> GMDEIVKNIREGTHVLLPFYETLPELNLSLGKSPLPSLEYGANYFLQISRVNDLNRMPTDMLKLFTHDIMLPESDLDKVYEILKINSVKYYGRTTRADAVVADLSARNKLFKRERDAIKSNNHLTENNLYISDYKMLTFDVFRPLFDFVNEKYCIIKLPTLFGRGVIDTMRIYCSLFKNVRLLKCVSDSWLKDSAIMVASDVYKKNLDLFMSHVKSVTKSSSWKDVNTVQFSILNDPVDTEFTNKFLEFSNRVYEALYYVHSLLYSSMTSDSKSIENK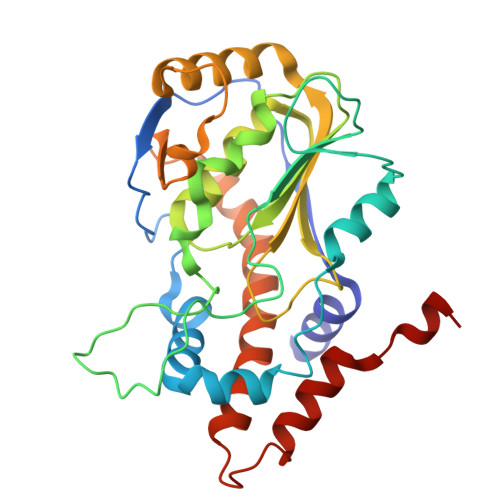HQRRLVKLLLHHHHHHHH>[4x]SNGGGMLWDYAQ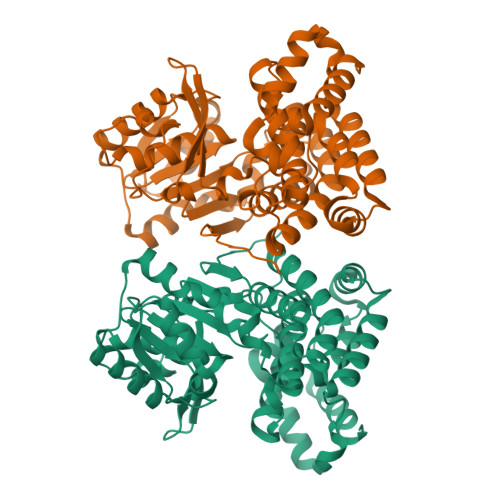PVTIRFGKGRAMEIKDIAEAMGLHDGIMVTPKFFVDSGEAQRLIDASDGAVSTVFTDFSPNPDVTEVDACAEIIRKNHCEFVVAMGGGSAMDVSKAAASICLTDDSIADYHGTGKAMPQKHLPIIALPTTAGTGSEVTCVSVLTNRKLGKKAPIVSDGFFPSVAIVDPELTYSVPPKITASTGMDVLSQAIEGFWSKGHQPICDSCAAHAAKLVFKYLPIAVAEPHNEEAREKMCEASVIAGLAFTLPKTTSSHACSFPLTNIHGIPHGEACGLTLDYFARINKDAQHGRVQEFARGIGFKDVDAMADAIHDLKVRIGMRTGLKDLNLTEEQIADLVRISRHPNLYNNPVEITDDMLDTMYHYLASTD> MKIYRPLWEDGAFLMPQQFQQQAAWDVHLADSVARMGLAHPWGVV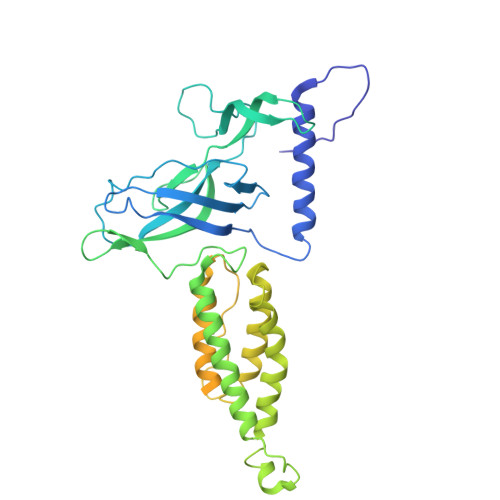AAEFDDSLLPLSRLNATRLIVRFPDGTLIDTERADNLPPVCDLSTVSDRSLVDIVLALPLLNANGGNLDNGSESERPRRWKSERVNVQELAGHEQSEVAVLRHNLTLRMAHQENAAWLTCPVTRLVRDAQGQWCRDPRFIPPLLTLSASPSLMTELLELLHHLQARRQRLMSMRRENNARLADFAVADVSLFWLLNALNSAEPVLKELLDMPYRHPELLYRELARLAGSLLTFSLEHNVDAVPAYHHETPENVFPPLLSLLNRLLEASLPSRVVFIELKQKGVMWEGALHDARLREGADFWLSVRSSMPGHELQTKFPQLCKAGSPDDVSEVVNVALSGVIIRPVTHVPAAIPLRLENQYFALDLSTDAARAMLDAGRCTFYTPASLGDVKLELFAVLR> MATTDKKDEENLRAYKFRLDPNQAQTTALYQAVGAARYTYNMLTAYNLEVNRLRDDYWKRRHDEDISDADIKKELNALAKEDKRYKQLNYGAFGTQYLTPEKKRHEQAEHRIENGEDPSVVWNQETERSANPWLHTANQRV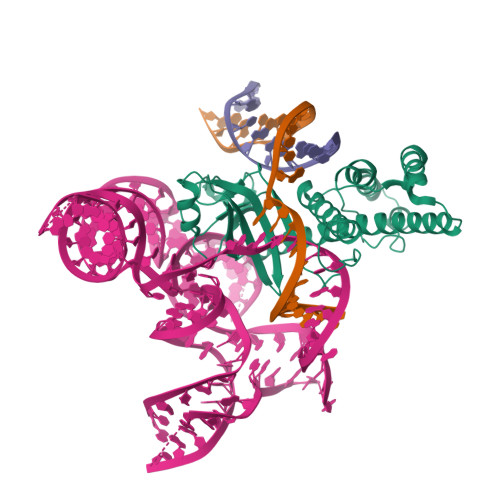LVSGLQNASDAWDNFWASRTGKRAGRLVGTPRFKKKGVSRDSFTVPAPEKMGAYGTAYLRGEPAYKQGRRKITDYRHVRLSYLGTIRTFNSTKPLVKAVVAGAKIRSYTVSRNADRWYVSFLVKFSEPIRRSATKRARAAGSVGVDLGVKYLASLSDSEAPQRFPNLKFVEGLPSLENPRWSEASSRRLHKLQRALARSQKGSNRRSRLVKQIARLHHMTALRRESNLHQLTKKLATEYTLVGFEDLNVSGMTASAKGTVENPGKNVAQKSGLNRVVLDAAFGVFRNQLEYKAVWYGSAFEKVDRYFASSQTCSECGRKAKTKLTLRDRVFDCAYCGNMMDRDLNAAVNICREAQRLFDEKLASEDRESLNGRGSRGALRGAETVEASRPPASHRRGSP>[2x]MRVLALSAVFLVASIIGMPAVAKEWQENKSWNAHFTEHKSQGVVVLWNENKQQGFTNNLKRANQAFLPASTFKIPNSLIALDLGVVKDEHQV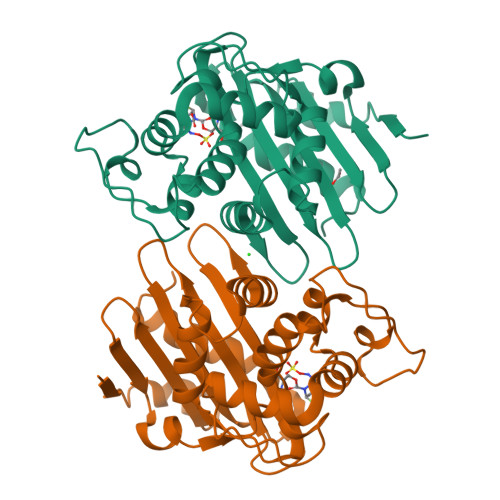FKWDGQTRDIATWNRDHNLITAMKYSVVPVYQEFARQIGEARMSKMLHAFDYGNEDISGNVDSFWLDGGIRISATEQISFLRKLYHNKLHVSERSQRIVKQAMLTEANGDYIIRAKTGYSTRIEPKIGWWVGWVELDDNVWFFAMNMDMPTSDGLGLRQAITKEVLKQEKIIP> GPHMGGSAEVNASPLKHFVTAKKKINGIFEQLGAYIQESATFLEDTYRNAELDPVTTEEQVLDVKGYLSKVRGISEVLARRHMKVAFFGRTSNGKSTVINAMLWDKVLPSGIGHTTNCFLRVEGTDGHEAFLLTEGSEEKRSAKTVNQLAHALHQDKQLHAGSLVSVMWPNSKCPLLKDDLVLMDSPGIDVTTELDSWIDKFCLDADVFVLVANSESTLMQTEKHFFHKVSERLSRPNIFILNNRWDASASEPEYMEEVRRQHMERCTSFLVDELGVVDRSQAGDRIFFVSAKEVL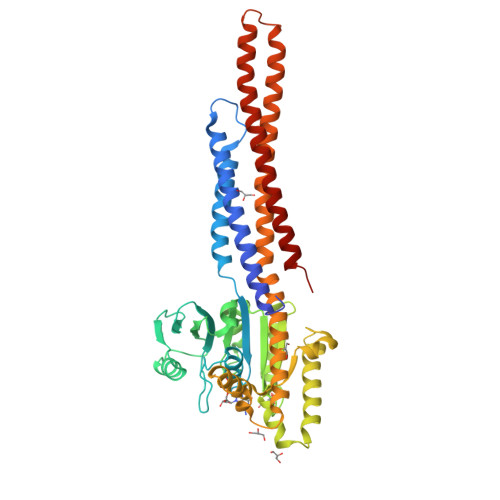NARIQKAQGMPEGGGALAEGFQVRMFEFQNFERRFEECISQSAVKTKFEQHTVRAKQIAEAVRLIMDSLHMAAREQQVYCEEMREERQDRTRENLEQEIAAMNKKIEVLDSLQSKAKLLRNKAGWLDSELNMFTHQYLQPSR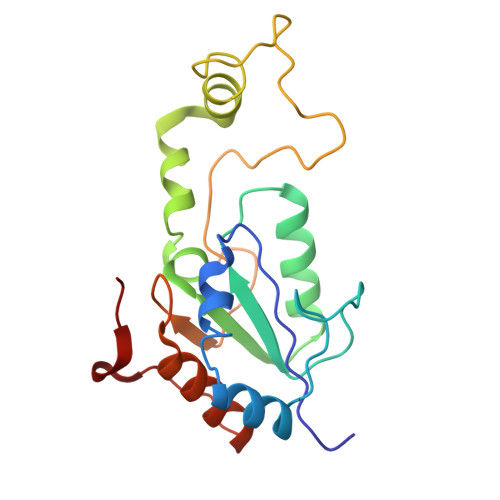> MAKAKVATFWLEACAGCHMSFLDLDERLIDLFQNVEILFSPIVDAKDIPNIDVGVLSGGLGNVEEVELAKKMRERCKYLVAWGDCAVFGGINCMRNFIPKDVVLREGYIETASTVNPQGIVPSEDIPELLPRALPIDYEVKVDVYVPGCPPDADTIYYVFKELLAGRVPKVPSEMMRYD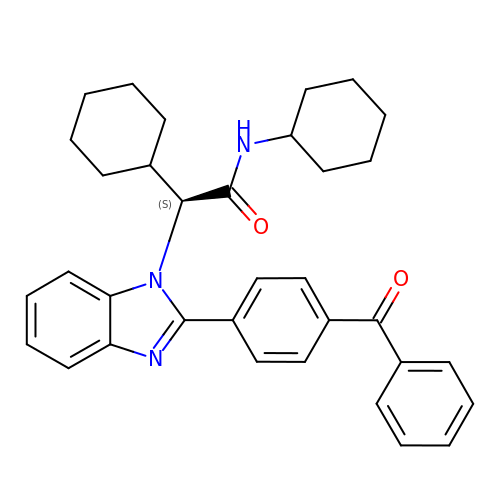(2S)-2-{2-[4-(benzenecarbonyl)phenyl]-1H-benzimidazol-1-yl}-N,2-dicyclohexylacetamide | C34 H37 N3 O2 | UYOADCMXWNRRPQ-HKBQPEDESA-N>MSERPKTLPPTLRDKKRYIAFKVISENQFNKDEIKEAIWNACLRTLGELGTAKAKPWLIKFDETTQTGIIRSDRNHVYDVIFSLTL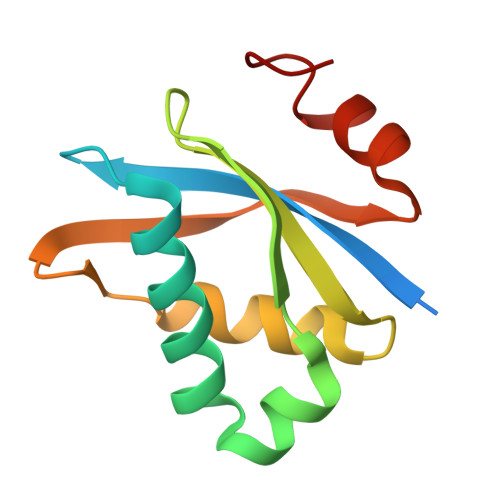VSDINGNKAIIKVLGVSGTIKRLKRKFLSQFGWR[5x]>[4x]QSVEESEGGLFKPTDTLTLTCTASGFSLSGHGVIWVRQAPGKGLEWIGSAGAYGRIYYASWAKSRSTITRNTNLNTVTLKMTSLTAADTATYFCARRSDVGTSVGFDSWGPGTLVTISSSSGQPKAPSVFPLAPCCGDTPSSTVTLGCLVKGYLPEPVTVTWNSGTLTNGVRTFPSVRQSSGLYSLSSVVSVTSSSQPVTCNVAHPATNTKVDKTVAPSTCSHHHHHH;>[4x]DMTQTPSSKSVPVGDTVTINCQASESVYSNNRLSWFQQKPGQPPKLLIYLVSTLASGVPSRFKGSGSGTQFTLTISDVVCDDAATYYCVGYKSSTTDGLAFGGGTEVVVKGDPVAPTVLIFPPAADQVATGTVTIVCVANKYFPDVTVTWEVDGTTQTTGIENSKTPQNSADCTYNLSSTLTLTSTQYNSHKEYTCKVTQGTTSVVQSFNRGDC;>RNIIXGSDS[4x]

Phosphohistidine (pHis) is a labile posttranslational modification with two isoforms, 1-pHis and 3-pHis, involved in many cellular processes across the kingdoms of life. Previously, we developed monoclonal antibodies (mAbs) against the 1-pHis and 3-pHis modifications using stable phosphotriazolylalanine mimetics as immunogens. Here, we report structures of Fab fragments derived from five rabbit pHis mAbs crystallized in complex with their cognate 1-pTza and 3-pTza peptides. These structures provide critical information about the molecular mechanism of phosphoepitope recognition, isomer specificity, sequence independence, and noncross-reactivity to other phosphoamino acids.

In the 1-pHis Fabs the peptidyl phosphate is oriented toward the CDRH2 loop, whereas it is anchored on CDRH3 in the 3-pHis antibodies thus creating a deeper pocket. In the SC1-1:NM23-1-pTza, the peptidyl phosphate group forms hydrogen bonds with the main-chain amide of Ala53 and the side-chain hydroxyl group of Tyr58 in CDRH2. Arg95 in CDRH3 undergoes a bidentate salt bridge with the phosphate group. An additional hydrogen bond is contributed by the hydroxyl group of Ser94 in the CDRL3 loop. The auxiliary interactions are mediated by two water molecules sequestered in the binding site. The key feature of phosphate binding by the 1-pHis Fabs is the participation of Arg95 in CDRH3 loop in forming salt bridges with the phosphate; this type of phosphate interaction is shared with two phosphate-binding superfamilies, FMN-linked oxidoreductases and PRTase, as well as SH2 and PTB domain-containing proteins that recognize pTyr modifications. The bound peptides adopt a type I β-turn conformation around residues I-1-pTza-GS. In the case of SC1-1:NM23-1-pTza, Tyr91 and Ser94 in CDRL3 make hydrogen-bond interactions with amide and carbonyl backbone atoms of two residues on the peptide, respectively. However, the direct and water-mediated hydrogen bonds formed with the N3 (N3 equivalent in imidazole ring of His) in 1-pHis Fabs and N2 (N1 equivalent in imidazole ring of His) in 3-pHis Fabs means the topography of the CDR can exclude nonisoform specific substrate binding.>SNAMSQLVTHAFDDATALSFDGRQFHGQVKAEYYNMVGPFGGITAATMLK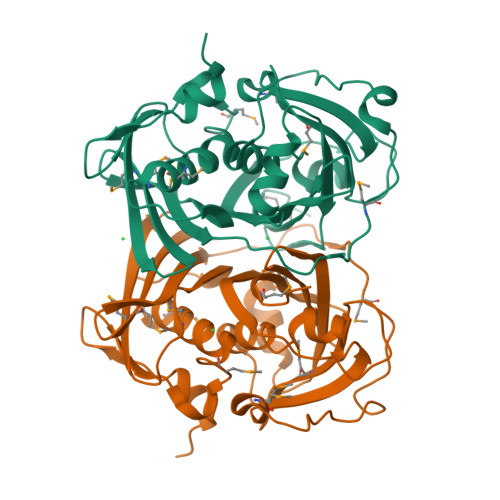AAMSHPERLGQPLALTVNFAAPAKVAPFVIEAVPVRTNRSTQHFTLTMMQDGEVVTTATAVFGIRRESWSHTEAVMPDVPPPADVPRFVAPAPLPWMQWYHVRLIRGSAFDEVQDATTYQWMRDDPPRPLDHAALAALCDTFVPRVYVKLKRPVPIGTVTFTVYFLADPETIFRQGTNELLGVARATGFSHGYFDQIGEVWSQDGDLLATTTQLVYMKAPVSGSS[2x]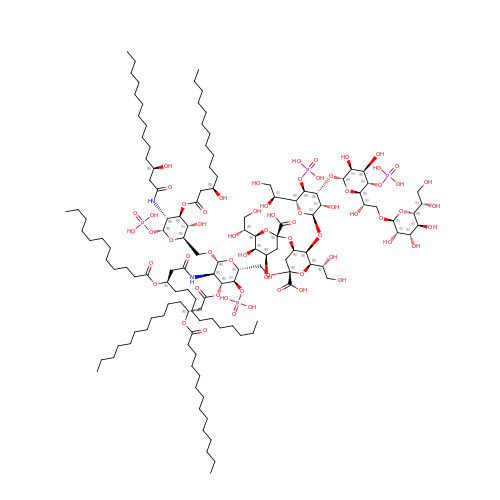(2~{R},4~{R},5~{R},6~{R})-6-[(1~{R})-1,2-bis(oxidanyl)ethyl]-2-[(2~{R},4~{R},5~{R},6~{R})-6-[(1~{R})-1,2-bis(oxidanyl)ethyl]-5-[(2~{S},3~{S},4~{R},5~{R},6~{R})-6-[(1~{S})-1,2-bis(oxidanyl)ethyl]-4-[(2~{R},3~{S},4~{R},5~{S},6~{R})-6-[(1~{S})-2-[(2~{S},3~{S},4~{S},5~{S},6~{R})-6-[(1~{S})-1,2-bis(oxidanyl)ethyl]-3,4,5-tris(oxidanyl)oxan-2-yl]oxy-1-oxidanyl-ethyl]-3,4-bis(oxidanyl)-5-phosphonooxy-oxan-2-yl]oxy-3-oxidanyl-5-phosphonooxy-oxan-2-yl]oxy-2-carboxy-2-[[(2~{R},3~{S},4~{R},5~{R},6~{R})-5-[[(3~{R})-3-dodecanoyloxytetradecanoyl]amino]-6-[[(2~{R},3~{S},4~{R},5~{R},6~{R})-3-oxidanyl-5-[[(3~{R})-3-oxidanyltetradecanoyl]amino]-4-[(3~{R})-3-oxidanyltetradecanoyl]oxy-6-phosphonooxy-oxan-2-yl]methoxy]-3-phosphonooxy-4-[(3~{R})-3-tetradecanoyloxytetradecanoyl]oxy-oxan-2-yl]methoxy]oxan-4-yl]oxy-4,5-bis(oxidanyl)oxane-2-carboxylic acid | C131 H240 N2 O63 P4 | MVYTXVAKEAWEGM-SMTLFHDCSA-N> SRPAVLSDIQPYVPRYCGNLANSDAPETVNKLSVDSKNELTIDTRTMGLGGADELTIHSIASRMTFWRQFDWPESAVTDTLLASMSVQPFCIDTVTASPVTEI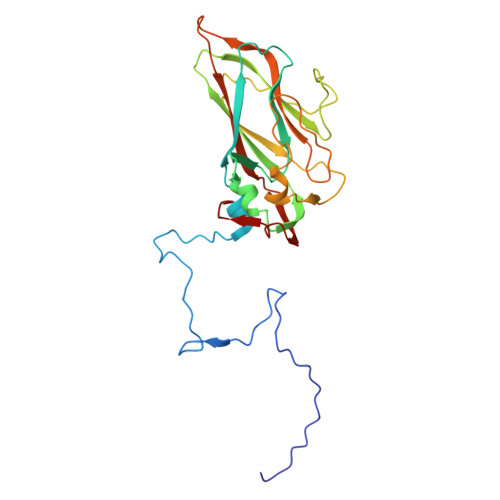HSTALAFASAPFETWQGSIKFHFKVVCSEYHRGRLRLVYNPLTNNAGPVAFNQVYSTTIDISNDREFDYECKWTDIRAWNACIGIDGATSATFFNTAAAVTGGTPFDNGTLSVYVVNELATPSTAAADVKVQVWVSAGDDFAVAVPGVGLSQLSYFQQQ>[3x]ASNFTQFVLVDNGGTGDVTVAPSNFAN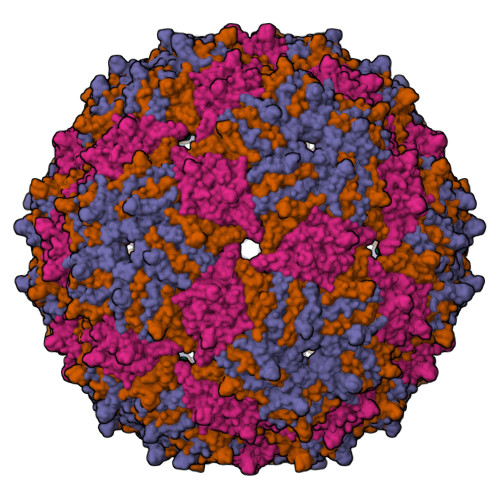GVAEWISSNSRSQAYKVTCSVRQSSAQNRKYTIKVEVPKVATQTVGGVELPVAAWRSYLSMELTIPIFATNSDCELIVKAMQGLLKDGNPIPSAIAANSGIY>MSTPGAQQVLFRTGIAAVNSTNHLRVYFQDVYGSIRESLYEGSWANGTEKNVIGNAKLGSPVAATSKELKHIRVYTLTEGNTLQEFAYDSGTGWYNGGLGGAKFQVAPYSCIAAVFLAGTDALQLRIYAQKPDNTIQ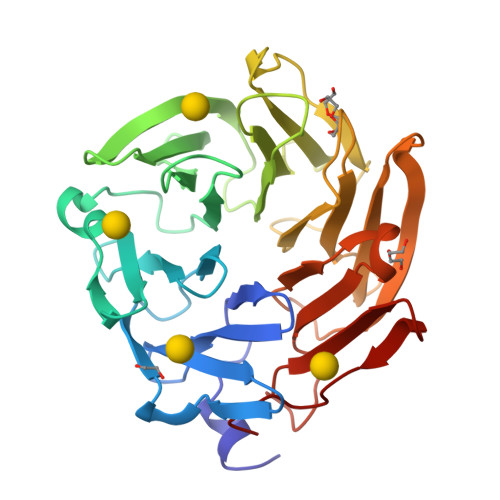EYMWNGDGWKEGTNLGGALPGTGIGATSFRYTDYNGPSIRIWFQTDDLKLVQRAYDPHKGWYPDLVTIFDRAPPRTAIAATSFGAGNSSIYMRIYFVNSDNTIWQVCWDHGKGYHDKGTITPVIQGSEVAIISWGSFANNGPDLRLYFQNGTYISAVSEWVWNRAHGSQLGRSALPPA[4x]>GPHMVRKQEIIKVNQQLIEAISNGDFESYTKMCDPGMTAFEPEALGNLVEGLDFHRFYFENLWSRNSKPVHNTMLNPHIHLMGDESAC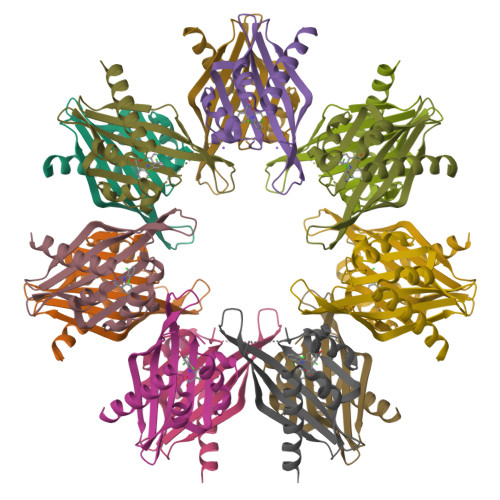IAYIRITQYLDAGGIPRTAQSEETRVWHRRDGKWQHVHMHRSGAPSV[7x]> MAGPCYNPNEHYLPASFKGVPFDADSSDSEHGRNGAEAEFVFGERTGYADLGIKIRSYSIRARFQTNDHVALSNAFIAVLESTGPGLLVHPTRGPVMAACRSARVTDSKVDAAGVTYIDIDFVEANDTVTGFGLVGSLIALALSPIITATEESFKRYYSPENVRYYNSETVIATMAEAVQQVQTGYLALSGNDTSQEKWTIVRDFRNVLIDEFTFFDPANSWNVLRNGFSYLDSAAVGQDKFTILRNIINWSSSHSELDGESADAQNAIFSAVRVLATAYLSKAYMETVASTVNEGLAQYDQIAAILEQEAQIAQEDCHDNEFFLSIREFSVSVARVMVNRAYNSPALIVY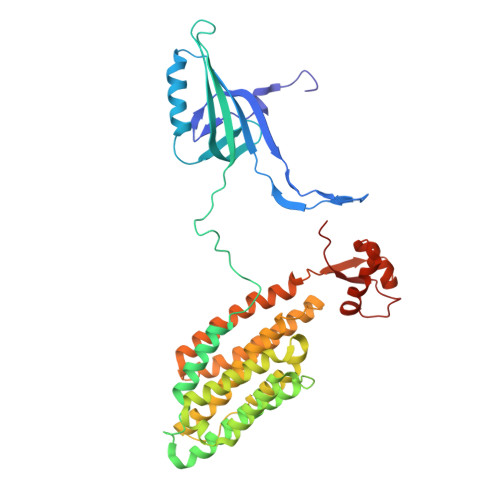SFPGTMHSLVVAWEIFGDAKRSRELEGRNTGAPWAIGPKVIAERVRA>[2x]APLADAALPEPNVFLIFSHGLQGCLEAQGGQVRVTPACNTSLPAQRWKWVSRNRLFNLGTMQCLGTGWPGTNTTASLGMYECDREALNLRWHC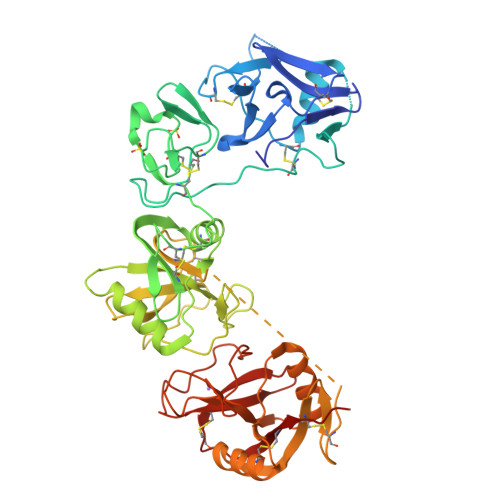RTLGDQLSLLLGARTSNISKPGTLERGDQTRSGQWRIYGSEEDLCALPYHEVYTIQGNSHGKPCTIPFKYDNQWFHGCTSTGREDGHLWCATTQDYGKDERWGFCPIKSNDCETFWDKDQLTDSCYQFNFQSTLSWREAWASCEQQGADLLSITEIHEQTYINGLLTGYSSTLWIGLNDLDTSGGWQWSDNSPLKYLNWESDQPDNPSEENCGVIRTESSGGWQNRDCSIALPYVCKKKPNATAEPTPPDRWANVKVECEPSWQPFQGHCYRLQAEKRSWQESKKACLRGGGDLVSIHSMAELEFITKQIKQEVEELWIGLNDLKLQMNFEWSDGSLVSFTHWHPFEPNNFRDSLEDCVTIWGPEGRWNDSPCNQSLPSICKKAGQLSG>SEFELGAPAGRQAGQQATVDRLRTQVTGFLSGALGKLQALSAQNMDPELAQFRVLDVDRAIMPLLIVAENARNPGLNLVPLHMDMAEDEEVRTQPPMAGSRHIAEFVASARPG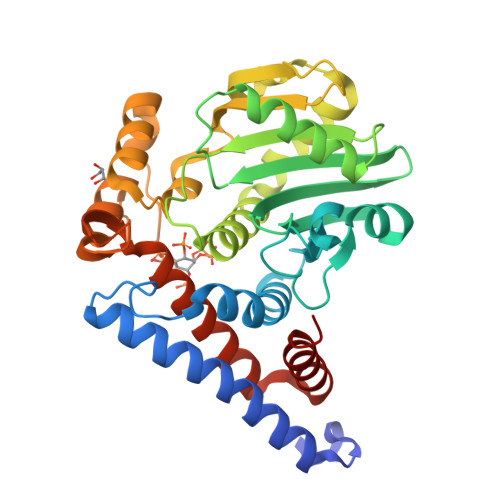RYRAVIDDGSHTRAADIRKDASGTSVIVVDPLRKEKDESAYVDYADNVNMEFGEHAKCAFIPVDIQKSFFDCRILSLSLALKMHDKDDAFAAFHETLRNGGDPSHHVSRAQQTEELGATLVLDGAPLVDARMMKHGQAASSVSRYLGNHPEQSTVPVNKRNETLGERTTRHLVKRKVRNRADSEGRVTSGETKEITFSNSVEQKRIALLNRAASYVNSAPPPVVMRMAKLLQDSLLDTN[4x]>MLNPIVRKFQYGQHTVTLETGMMARQATAAVMVSMDDTAVFVTVVGQKKAKPGQDFFPLTVNYQERTYAAGRIPGSFFRREGRPSEGETLIARLIDRPVRPLFPEGFVNEVQVIATVVSVNPQVNPDIVAMIGASAALSLSGIPFNGPIGAARVGYINDQYVLNPTQDELKESKLDLVVAGTEAAVLMVESEAELLSEDTMLGAVV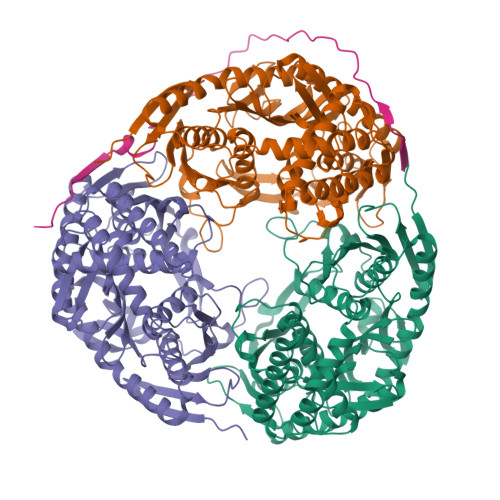FGHEQQQVVIQAINDLVKEAGKPRWDWQPEAVNDALNARVAALAESRLSDAYRITDKQERYAQVDVIKSETIEQLIAEDETLDANELGEILHAIEKNVVRSRVLAGEPRIDGREKDMIRGLDVRTGVLPRTHGSALFTRGETQALVTATLGTARDAQVLDELMGERTDSFLFHYNFPPYSVGETGMVGSPKRREIGHGRLAKRGVLAVMPDMDKFPYTVRVVSEITESNGSSSMASVCGASLALMDAGVPIKAAVAGIAMGLVKEGDNYVVLSDILGDEDHLGDMDFKVAGSRDGISALQMDIKIEGITKEIMQVALNQAKGARLHILGVMEQAINAPRG[3x];> NHASAPMTRAPAPEYVPETPHHSDWQRPSFHFEGKGAAGGHSATRHASAPATRPQPVE> MILDVDYITEEGKPVIRLFKKENGKFKIEHDRTFRPYIYALLRDDSKIEEVKKITGERHGKIVRIVDVEKVEKKFLGKPITVWKLYLEHPQDVPTIREKVREHPAVVDIFEYDIPFAKRYLIDKG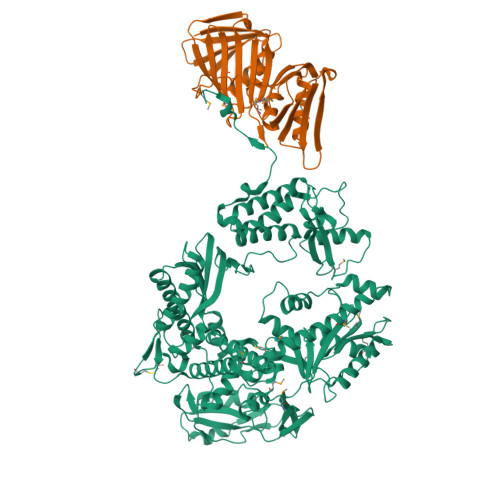LIPMEGEEELKILAFDIETLYHEGEEFGKGPIIMISYADENEAKVITWKNIDLPYVEVVSSEREMIKRFLRIIREKDPDIIVTYNGDSFDFPYLAKRAEKLGIKLTIGRDGSEPKMQRIGDMTAVEVKGRIHFDLYHVITRTINLPTYTLEAVYEAIFGKPKEKVYADEIAKAWESGENLERVAKYSMEDAKATYELGKEFLPMEIQLSRLVGQPLWDVSRSSTGNLVEWFLLRKAYERNEVAPNKPSEEEYQRRLRESYTGGFVKEPEKGLWENIVYLDFRALYPSIIITHNVSPDTLNLEGCKNYDIAPQVGHKFCKDIPGFIPSLLGHLLEERQKIKTKMKETQDPIEKILLDYRQKAIKLLANSFYGYYGYAKARWYCKECAESVTAWGRKYIELVWKELEEKFGFKVLYIDTDGLYATIPGGESEEIKKKALEFVKYINSKLPGLLELEYEGFYKRGFFVTKKRYAVIDEEGKVITRGLEIVRRDWSEIAKETQARVLETILKHGDVEEAVRIVKEVIQKLANYEIPPEKLAIYEQITRPLHEYKAIGPHVAVAKKLAAKGVKIKPGMVIGYIVLRGDGPISNRAILAEEYDPKKHKYDAEYYIENQVLPAVLRILEGFGYRKEDLRYQKTRQVGLTSWLNIKKS;> PFEIVFEGAKEFAQLIDTASKLIDEAAFKVTEDGISMRAMDPSRVVLIDLNLPSSIFSKYEVVEPETIGVNLDHLKKILKRGKAKDTLILKKGEENFLEITIQGTATRTFRVPLIDVEEMEVDLPELPFTAKVVVLGEVLKAAVKAASLVSDSIKFIARENEFIMKAEGETQEVEIKLTLEDEGLLDIEVQEETKSAYGVSYLSDMVKGLGKADEVTIKFGNEMPMQMEYYIRDEGRLTFLLAPRVEE>[2x]SMKEWQENKSWNAHFTEHKSQGVVVLWNENKQQGFTNNLKRANQAFLPASTFKIPNSLIALDLGVVKDEHQVFKWDGQTRDIATWNRDHNL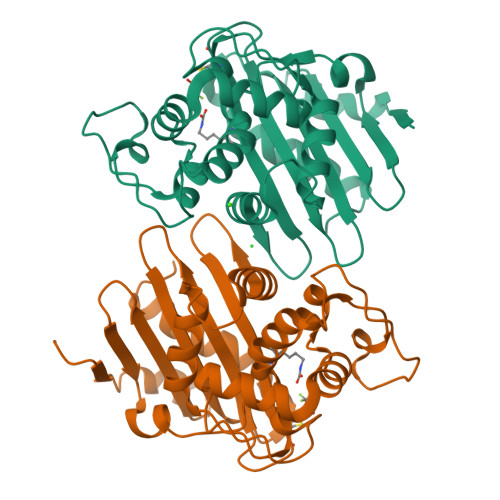ITAMKYSVVPVYQEFARQIGEARMSKMLHAFDYGNEDISGNVDSFWLDGGIRISATEQISFLRKLYHNKLHVSERSQRIVKQAMLTEANGDYIIRAKTGYSCRIEPKIGWWVGWVELDDNVWFFAMNMDMPTSDGLGLRQAITKEVLKQEKIIP>MATVEPETTPTPNPPTTEEEKTESNQEVANPEHYIKHPLQNRWALWFFKNDKSKTWQANLRLISKFDTVEDFWALYNHIQLSSNLMPGCDYSLFKDGIEPMWEDEKNKRGGRWLITLNKQQRRSDLDRFWLETLLCLIGESFDDYSDDVCGAVVNVRAKGDKIAIWTTECENREAVTHIGRVYKERLGLP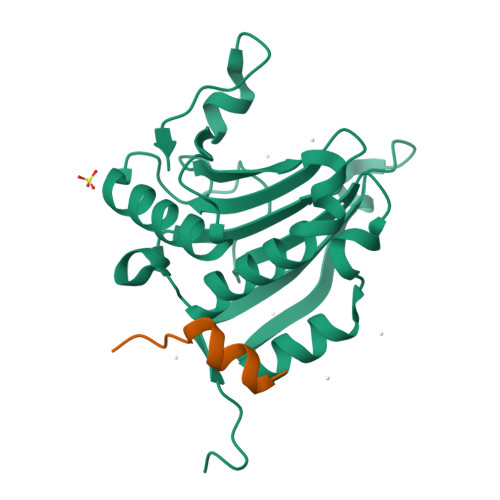PKIVIGYQSHADTATKSGSTTKNRFVV[2x];>[2x]PGGTRIIYDRKFLMECRNSP>[2x]GPHMETVPYQIPYTPSELEELQQNIKLELEGKEQELALELLNYLNEKGFLSKSVEEISDVLRCSVEELEKVRQKVLRLEPLGVCSKDVWEFLELQIEEIYPEEEEILKKALRDLKRGKKLKPEIK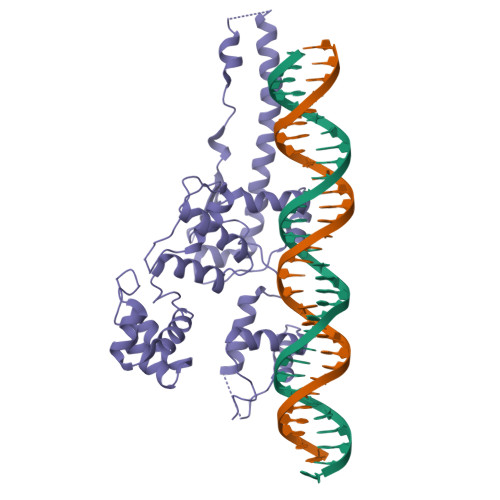GKLSRLRLFPLSSSAEKVYTFAKVDAIIEEENGEFFIYLYEDFIDIDLNEEYWELYKKSRNLQKELKEAFERYESIRKVLDIRRRNLRKVLEKIVERQKDFLTGKGSLKPLTLREVSSEIGIHESTLSRIVNSKYVKTPVGTYSLRTFFVRESAEGLTQGELMKLIKEIVENEDKRKPYSDQEIANILKEKGFKVARRTVAKYREMLGIPSSRERRI>PRGSMLELPPVASLKGKSITSAEQFSRADIYALIHLASAMQRKIDAGEVLNLLQGRIMTPLFFEDSSRTFSSFCAAMIRLGGSVVNFKVEASSINKGETLADTIRTLDSYSDVLVMRHPRQDAIEEALSVAQHPILNAGNGAGEHPTQALLDTLTIHSELGSVDGITIALIGDLKMGRTVHSLLKLLVRNFSIKCVFLVAPDALQMPQDVLEPLQHEIATKGVIIHRTHALTDEVMQKSDVLYTTRLQKERFMASTSDDAAAL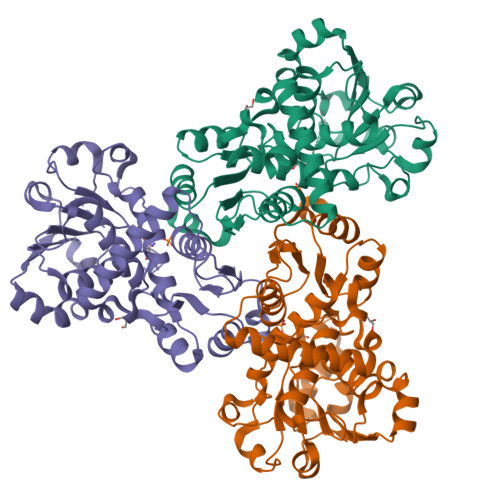QSFAAKADITIDAARMRLAKEKMIVMHPLPRNDELSTTVDADPRAAYFRQMRYGMFMRMAILWSVLA[6x]>GMGKRGREGTLDKARCLAFVHQLWDKDKLKMFHHPISAAELPDYHKVINYPVDLSTIRQGIESGKYDSDADVQNAVAQMIANALEYNAKGTEWHQQALSFRSIYLD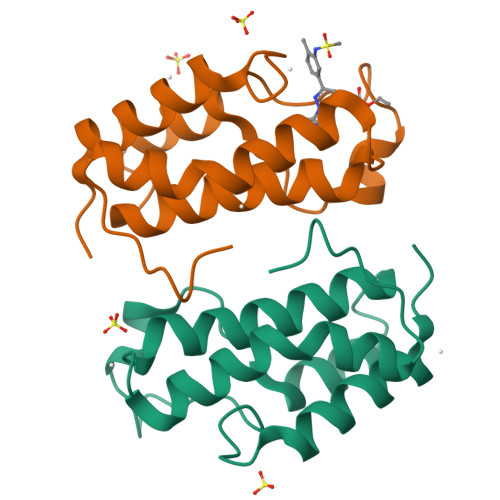VARQCGLSVDDDAAY[2x]>SHMASMPPYTVVYFPVRGRCAALRMLLADQGQSWKEEVVTVETWQEGSLKASCLYGQLPKFQDGDLTLYQSNTILRHLGRTLGLYGKDQQEAALVDMVNDGVEDLRCKYISLIYTNYEAGKDDYVKALPGQLKPFETLLSQNQGGKTFIVGDQISFADYNLLDLLLIHEVLAPGCLDAFPLLSAYVGRLSARPKLKAFLASPEYVNLP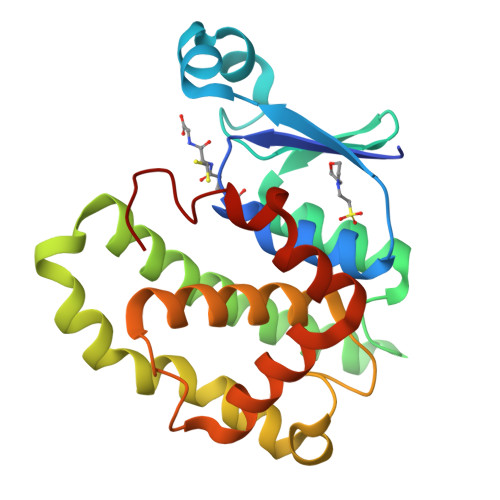INGNGKQ[2x]>MSLSIGRTCWAIAEGYIPPYGNGPEPQFISHETVCILNAGDE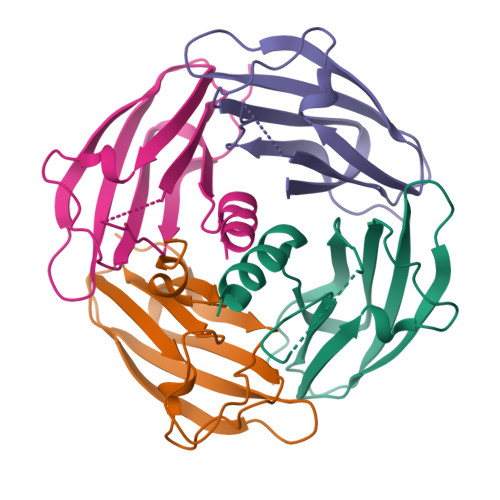DAHVEITIYYSDKEPVGPYRLTVPARRTKHVRFNDLNDPAPIPHDTDFASVIQSNVPIVVQHTRLDSRQAENALLSTIAYANTHHHHHH[8x]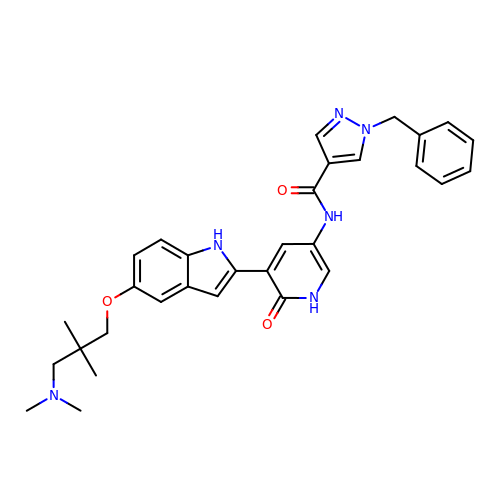1-benzyl-N-(5-{5-[3-(dimethylamino)-2,2-dimethylpropoxy]-1H-indol-2-yl}-6-oxo-1,6-dihydropyridin-3-yl)-1H-pyrazole-4-carboxamide | C31 H34 N6 O3 | REQMZUHAMVOEON-UHFFFAOYSA-N> MGSDKIHHHHHHENLYFQGMTLEARIEALEKEIQRLNDIEAIKQLKAKYFRCLDGKLWDELETTLSPNIETSYSDGKLVFHSPKEVTEYLAAAMPKEEISMHMGHTPEITIDSENTATGRWYLEDNLIFTDGKYKNVGINGGAFYTDKYEKIDGQWYIKETGYVRIFEE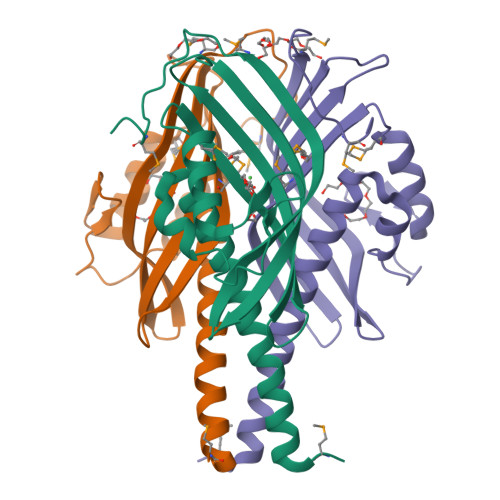HFMRDPKIHITSNMHKEK Neurospora crassa FRH (frequency-interacting RNA helicase) is a 124 kDa homolog of Saccharomyces cerevisiae Mtr4 (56% sequence identity, 73% similarity), a Ski2-like ATP-dependent RNA helicase that plays a central role in activating the nuclear exosome to promote processing or complete degradation of RNA substrates. FRH has been extensively characterized as an essential component of the circadian clock in N. crassa, a function which doesn’t exist in S. cerevisiae and is not dependent on enzymatic activity. Like previously determined structures of Mtr4 from Saccharomyces cerevisiae, FRH contains a largely unstructured (169 amino acid) N-terminus and five structured domains: two RecA-like domains, a small winged helix domain, a helical “ratchet” or DSHCT domain, and an arch-like insertion domain that includes a KOW module. The domain is composed of two anti-parallel alpha helical coiled coil segments (arm and forearm) that terminate with a β-barrel fold (fist) containing a KOW module.

The purified protein was crystallized in the presence of 0.2 M Sodium Citrate pH 5.6 and 19% PEG 3350, resulting in a trigonal P3121 crystal form (FRHTrig) that is unique from the previously published orthorhombic P212121 FRH structures (FRHOrtho). The newly determined FRHTrig structure retains the same general architecture as the previously determined FRHOrtho structures. In the FRHTrig structure, the RecA domains open slightly (12° rotation, 2.5 Å translation) with respect to each other as compared to the FRHOrtho structure. Furthermore, rearrangements in the ATP binding site in RecA1 result in a conformation that is consistent with productive nucleotide binding and hydrolysis as observed in nucleotide bound Mtr4 structures. Thus, the FRHTrig structure appears to be more representative of the native nucleotide binding conformation. (3) The most prominent difference between the two FRHTrig and FRHOtrho structures is the conformation of the arch domain. Rotations about multiple hinge points in the arch result in a 30 Å displacement and a 70° rotation of the KOW module with respect to the FRHOrtho small cell position. Hinge points are observed (1) at the base of the arch where it projects out from the winged helix domain, (2) at the junction between the arm and the forearm, and (3) at the junction between the forearm and the fist (containing the KOW module). Symmetry related regions along the elbow, forearm and fist/KOW of the arch domain interlock to stabilize the extended conformation of the arch domain, including the 70° rotation of the fist/KOW (as compared to the FRHOrtho structures). We conclude that FRH is a monomer in solution and the structural dimer observed in the FRHTrig crystal is likely a crystallization artifact, although we cannot rule out the possibility that such a conformation may be biologically relevant under some conditions not yet identified.

> MDDLFEVFEEQPRAQKKRKASPDVEMADGAAAAAPVANAAAAVTHPQAQAAPAPQKDNIDNNDNNNNNTTTSAVQPTIPNGDAAAAADDVQSPQSPHGLGDNKRRKKTDEAEPIMTDAFQTAESREVTGAQGFAPTEGESIVLSHNIQHQVALPPDLDYEYIPLSEHKPPAEPARTYSFKLDPFQALSVASIEREESVLVSAHTSAGKTVVAEYAIAQCLKKNQRVIYTSPIKALSNQKYRDFQAEFGDVGLMTGDVTINPTASCLVMTTEILRSMLYRGSEIMREVAWVVFDEIHYMRDKIRGVVWEETIILLPDKVRYVFLSATIPNAFQFAEWIAKIHRQACHVVYTDFRPTPLQNYFFPAGGKGILLIVDEKGNFKENNFNQAMAMIEEKKGTDSNDWSAKQKGKGKNKKTNKGGEAADEKADIAKIIKMILKKNFQPVIVFNFSKRECEQMALASSSMKFNAPDEENMVNKVFENALASLSEDDKNLPQISNILPLLRKGIGVHHSGLLPILKETIEILFQEGLIKVLFATETFSIGLNMPARTVVFTQVTKWDGQQRRPLTSSEYIQMAGRAGRRGLDDRGIVIMMVDDKLEPETARAIVVGNQDKLNSAFHLGYNMVLNLLRIEAISPEYMLERCFFQFQNAASVPQLERELISLQQERDAIIIPDESIVKDYYGVRQQLEEYNKDMVFVIQHPQNCLGFFQEGRLIHIKSPSGVDYGWGVLIKHIQRQTPKNGQPPYPEQESYVLDVLLKVSGDFNPKTRGEGPMPEGIMPAGKDSKNARWEVVPCLLNCLRALGQLRVFLPKRLESADEKDGVGKAVDEISRRFPDGIPILDPMENMGINDDSFKKLLRKIEVLESRLVANPLHNSPLLVELWNQYSLKMQLGEQIKEKKKAIARAHSVAQLDELKSRKRVLRRLGFINDAEVVQMKARVACEISSTEGHELLLAELLFNRFFNELSPEICACILSCFIFDEKIETQALKEELAKPFREIQAQARIIAKVSAESKLDVNEDEYVQSLKWQLMETVLAWAQGRPFSEICKMTNVYEGSLIRLFRRLEELLRQMAEAARVMGSEELKDKFELSLSKIRRDIVSFNSLYL> MGHHHHHHQFVAWCREEASVTAGLPNVSELVDMVYEYCRKRGLYPDAESYPWKSNAHYWLVTN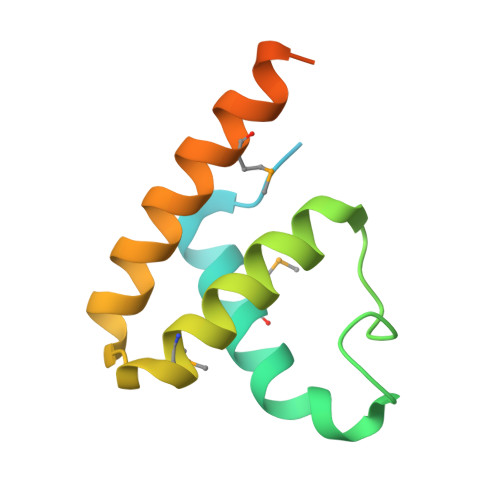LYQNMRANALTDAELRRKAADELVHMTARINRGEAIPEPVKQLPVMGGRPL In such microorganisms, the majority of small molecules are taken up by members of the OprD outer membrane protein family. Here we show that OprD channels require a carboxyl group in the substrate for efficient transport, and based on this we have renamed the family Occ, for outer membrane carboxylate channels. As expected from pairwise sequence identities that range from 35%–50%, the Occ proteins share a similar architecture, with a slightly off-center constriction formed by the inward-folded extracellular loops L3 and L7 and residues in the barrel wall. The transport data demonstrate that Occ channels have a pronounced preference for substrates with a carboxyl group, due to the universal presence of a basic ladder on one side of the barrel wall.

To determine if the phylogenetic subdivision of Occ proteins exists at the structural level, we determined X-ray crystal structures for seven Occ family members (OccD2, OccD3, and OccK2–K6). In fact, OccD2 (formerly OpdC) is closed in the crystal structure. Interestingly, the closed state of the OccD2 channel observed in the crystal structure features a strong interaction between the carboxyl group of Asp294 and the side chain of the central basic ladder residue Arg389. We speculate that the carboxylate in this interaction mimics that of the substrate during transport. For example, the dominant states of OccD1 and OccD2 have very small conductance values (∼15 pS), in accordance with the small/closed pores observed in the crystal structures. Interestingly, both channels show occasional upward spikes in conductance, suggesting the occurrence of infrequent gating events that form a larger pore. Indeed, we crystallized such a closed state for OccD2. All OccD channels, with the exception of OccD4, show good levels of arginine uptake. Thus, remarkably, OccD2 and OccD3, while efficient in arginine uptake, are not uptake channels for carbapenems. OccD channels are highly specific and transport basic amino acids.

>[4x]DEGEAKEGFIEGSSLQLLTRNYYFNHDRRHASGHDSKEWAQGFIATFQSGYTPGVVGFGVDAYGMLGLKLDGGGGTGGTSILPITSPSKEGYESGKAPDEFSSGGAALKIRAFDTELKLGDQFLSNPVVAGGESRMLPQTFRGVSLTNNSFEDLTLTAGQVSFTKYYNQSGHRRLGSYYGELPGDRDSHHLSWLGGTWGGIEGFTSSLYAAELQNVWKQYYADVDYTYEIDDNWSLNPGAHYYKTVDSGDSLLGRIDNNTYSLHFAVGYRQHTVTAVLQKVNGNTPFDYINQGDSIFLDNSQQYSDFNGPNEKSWKLQYDYDFVALGVPGLSASASYSRGKLDLTRVDPDSPGYGGWYSADGKNAKHWERDLDLQYVVQGGPAKDLSLRLRWATHRGTGGYSAVDNDIDEYRVIVDYPIDVFGGHHHHHH> MTMDEQQSQAVAPVYVGGFLARYDQSPDEAELLLPRDVVEHWLHAQGQGQPSLSVALPLNINHDDTAVVGHVAAMQSVRDGLFCLGCVTSPRFLEIVRRASEKSELVSRGPVSPLQPDKVVEFLSGSYAGLSLSSRRCDDVEQATSLSGSETTPFKHVALCSVGRRRG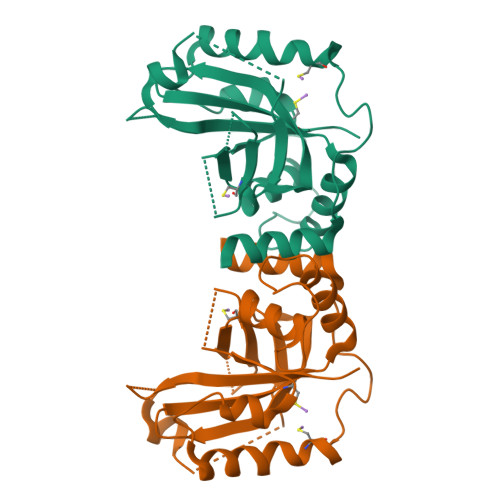TLAVYGRDPEWVTQRFPDLTAADRDGLRAQWQRCGSTAVDASGDPFRSDSYGLLGNYVDALYIRERLPKLRYDKQLVGVTERESYVKA> MTAGYEPCWLRYERKDQYSRLRFEEIVAKRTSPIFQAVVEELQKGLRSMMEIEPQVVQEVNETANSIWLGTLEDEEFERPLEGTLVHPEGYVIRSDVDDGPFRIYIIGKTDAGVLYGVFHFLRLLQMGENIAQLSIIEQPKNRLRMINHWDNMDGSIERGYAGRSIFFVDDQFVKQNQRIKDYARLLASVGINAISINNVNVHKTETKLITDHFLPDVAEVADIFRTYGIKTFLSINYASPIEIGGLPTADPLDPEVRRWWKETAKRIYQYIPDFGGFVVKADSEFRPGPFTYGRDHAEGANMLAEALAPFGGLVIWRCFVYNCQQDWRDRTTDRAKAAYDHFKPLDGQFRENVILQIKNGPMDFQVREPVSPLFGAMPKTNQMMEVQITQEYTGQQKHLCFLIPQWKEVLDFDTYAKGKGSEVKKVIDGS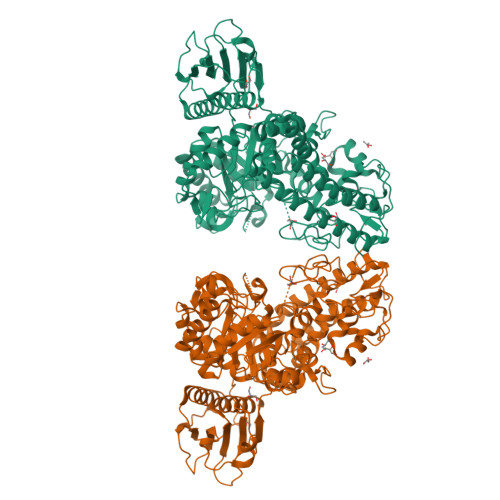LFDYRYSGIAGVSNIGSDPNWTGHTLAQANLYGFGRLAWNPDLSAEEIANEWVVQTFGDDSQVVETISWMLLSSWRIYENYTSPLGVGWMVNPGHHYGPNVDGYEYSHWGTYHYADRDGIGVDRTVATGTGYTAQYFPENAAMYESLDTCPDELLLFFHHVPYTHRLHSGETVIQHIYNTHFEGVEQAKQLRKRWEQLKGKIDEKRYHDVLERLTIQVEHAKEWRDVINTYFYRKSGIDDQYGRKIYR>[2x]FNEPLNIVSHLNDDWFLFGDARSDCTYVENNGHPKLDWLDLDPKLCNSGRISAKSGNSLFRSFHFIDFYNYSGEGDQVIFYEGVNFSPSHGFKCLAYGDNKRWMGNKARFYARVYEKMAQYRSLSFVNVSYAYGGNAKPTSICKDKTLTLNNPTFISKESNYVDYYYESEANFTLQGCDEFIVPLCVFNGHSKGSSSDPANKYYTDSQSYYNMDTGVLYGFNSTLDVGNTVQNPGLDLTCRYLALTPGNYKAVSLEYLLSLPSKAICLRKPKSFMPVQVVDSRWNSTRQSDNMTAVACQLPYCFFRNTSADYSGGTHDVHHGDFHFRQLLSGLLYNVSCIAQQGAFVYNNVSSSWPAYGYGHCPTAANIGYMAPVCIYDSDPLVPR

Murine coronaviruses, however, occur in two closely related biotypes that differ in HE ligand/substrate preference. One of these -represented by mouse hepatitis virus (MHV) strain DVIM- displays the presumptive ancestral specificity and targets 9-O-Ac-Sias, while the other -represented by MHV strain S- appears to have evolved to use 4-O-Ac-Sias instead (for supplementary introduction see Text S1 and Figure S1). We now present the crystal structure of the MHV-S HE receptor-binding domain, both in its native state and in complex with a receptor analogue. In overall structure, the HE of MHV-S closely resembles that of BCoV-Mebus. It assembles into homodimers and the monomers are composed of three modules: a small membrane-proximal (MP), a receptor-binding (R), and a central esterase (E) domain.

Crystals of free MHV-S HE and of a complex of HE0 with αNeu4,5Ac22Me diffracted to 2.1 and 2.5 Å resolution, respectively. The structure of the R domain, however, was resolved, and in the complex the ligand molecule is well-defined. While the overall organization of the MHV-S RBS is similar to that of BCoV-Mebus HE, the orientation of the receptor analogue with respect to the RBS is strikingly different. As compared to the ligand in the BCoV-Mebus HE binding site, the αNeu4,5Ac22Me receptor analogue is rotated by about 90° and shifted by about 2.5 Å. Two hydrogen bonds are formed between the nitrogen and oxygen main-chain atoms of Lys217 and the oxygen of the C4 acetyl group and the nitrogen of the 5-N-acetyl group, respectively. The Ser220 main chain nitrogen accepts an additional, weak hydrogen bond from the C8 hydroxyl group of the ligand. Most remarkably, the hydrophobic pocket that in BCoV-Mebus HE accommodates the 9-O-acetyl moiety of the receptor (comprised of Leu161, Tyr184 Leu266 and Leu267) -arguably the most crucial element of the BCoV HE RBS- is conserved in MHV-S HE (comprised of Ile166, Tyr189, Tyr281, and Leu282), but it now accepts the Sia 5-N-acetyl group, while the Sia glycerol side-chain is solvent exposed. Moreover, the hydrophobic patch in the BCoV-Mebus HE RBS that interacts with the Sia 5-N-acetyl group apparently changed into a shallow pocket that accommodates the Sia 4-O-acetyl moiety. As the Sia-4-O-acetyl group is crucial for ligand recognition by MHV-S HE, this pocket must be key to receptor-binding. In accordance, single Ala substitutions of Leu119, Ile166, Phe212, Leu260, or Tyr281 all reduced receptor-binding activity (although that of Ile166 to lesser extent) as shown by hemagglutination assay and solid-phase lectin binding assay.>[60x]MNIIKANVAAPDARVAITIARFNQFIND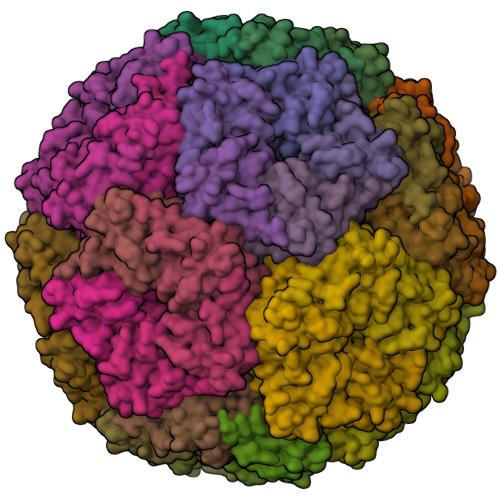SLLDGAVDALTRIGQVKDDNITVVWVPGAYELPLATEALAKSGKYDAVVALGTVIRGGTAHFEYVAGGASNGLASVAQDSGVPVAFGVLTTESIEQAIERAGTKAGNKGAEAALTALEMINVLKAIKA> 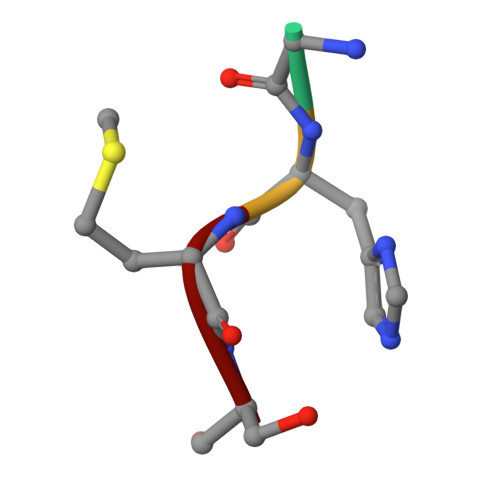GHMS> SGETSVPPGSALVGPSCVMDDFRDPQRWKECAKQGKMPCYFDLIEENVYLTERKKNKSHRDIKRMQCECTPLSKDERAQGEIACGEDCLNR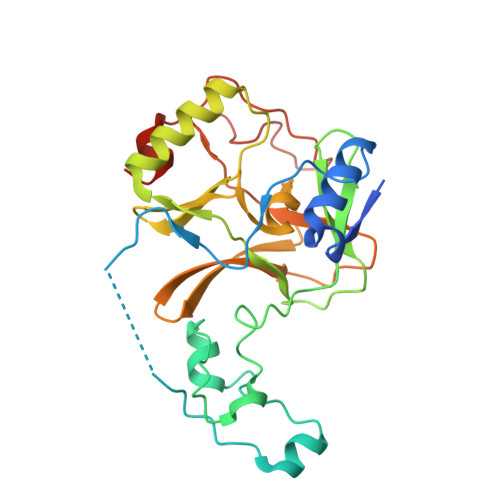LLMIECSSRCPNGDYCSNRRFQRKQHADVEVILTEKKGWGLRAAKDLPSNTFVLEYCGEVLDHKEFKARVKEYARNKNIHYYFMALKNDEIIDATQKGNCSRFMNHSCEPNCETQKWTVNGQLRVGFFTTKLVPSGSELTFDYQFQRYGKEAQKCFCGSANCRGYLGGENRVSIRAAGGKMKKERSRK> MDWKKIYEDRTCTADEAVKSIKSGDRVLFAHCVAEPPVLVEAMV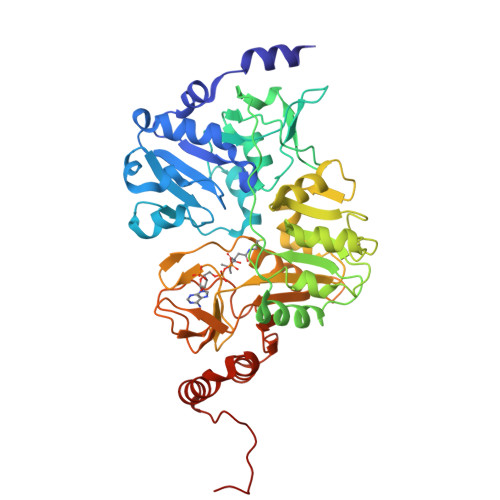ANAAAYKNVTVSHMVTLGKGEYSKPEYKENFTFEGWFTSPSTRGSIAEGHGQFVPVFFHEVPSLIRKDIFHVDVFMVMVSPPDHNGFCCVGVSSDYTMQAIKSAKIVLAEVNDQVPVVYGDTFVHVSEIDKFVETSHPLPEIGLPKIGEVEAAIGKHCASLIEDGSTLQLGIGAIPDAVLSQLKDKKHLGIHSEMISDGVVDLYEAGVIDCSQKSIDKGKMAITFLMGTKRLYDFAANNPKVELKPVDYINHPSVVAQCSKMVCINACLQVDFMGQIVSDSIGTKQFSGVGGQVDFVRGASMSIDGKGKAIIAMPSVAKKKDGSMISKIVPFIDHGAAVTTSRNDADYVVTEYGIAEMKGKSLQDRARALINIAHPDFKDELKAEFEKRFNAAFSAWSHPQFEK> GGACAUAUA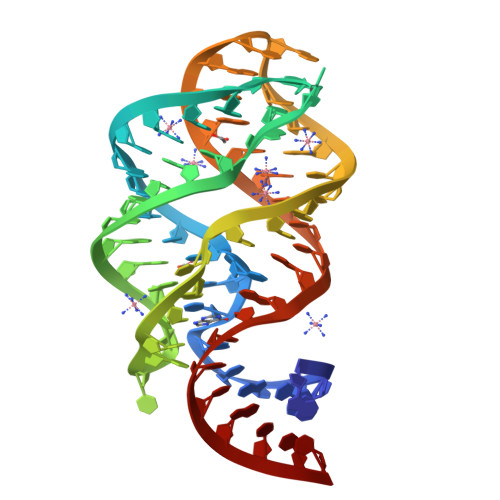UUCGCGUGGAUAUGGCACGCAAGUUUCUACCGGGCACCGUAAAUGUCCGACUAUGUCC> MSKVDLWQDATAQAELVRSGEISRTELLEATIAHVQAVNPEINAVIIPLFEKARRESELASGPFAGVPYLLKDLTVVSQGDINTSSIKGMKESGYRADHDAYFVQRMRAAGFVLLGKTNTPEMGNQVTTEPEAWGATRNPWNLGRSVGGSSGGSGAAVAAALSPVAHGNDAAGSVRIPASVCGVVGLKPTRGRISPGPLVTDSDNVAGAAHEGLFARSVRDIAALLDVVSGHRPGDTFCAPTASRPYAQGISENPGSLRVGVLTHNPVGDFALDPECAAAARGAAAALAALGHDVNDAYPEALGDRSFLKDYSTICDVAIA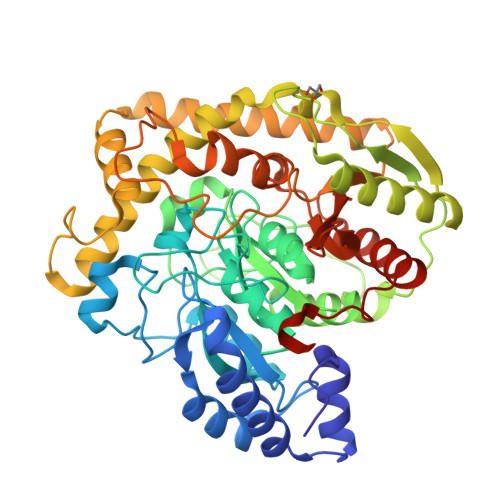REIERNGELIGRPLTEDDVEWTSWEMVKRADQVTGRAFAACVDELRYYAGKVERWWEAGWDLLILPTVTRQTPEIGELMLAKGTDLEGRQSAFISGSLQMLAFTVPFNVSGQPAISLPIGMSSDGMPIGVQIVAAYGREDLLLQVAAQLEGALPWVARRPQLLNPSRKIPAA> MEPSSKKLTGRLMLAVGGAVLGSLQFGYNTGVINAPQKVIEEFYNQTWVHRYGESILPTTLTTLWSLSVAIFSVGGMIGSFSVGLFVNRFGRRNSMLMMNLLAFVSAVLMGFSKLGKSFEMLILGRFIIGVYCGLTTGFVPMYVGEVSPTALRGALGTLHQLGIVVGILIAQVFGLDSIMGNKDLWPLLLSIIFIPALLQCIVLPFCPESPRFLLINRNEENRAKSVLKKLRGTADVTHDLQEMKEESRQMMREKKVTILELFRSPAYRQPILIAVVLQLSQQLSGINAVFYYSTSIFEKAGVQQPVYATIGSGIVNTAFTVVSLFVVERAGRRTLHLIGLAGMAGCAI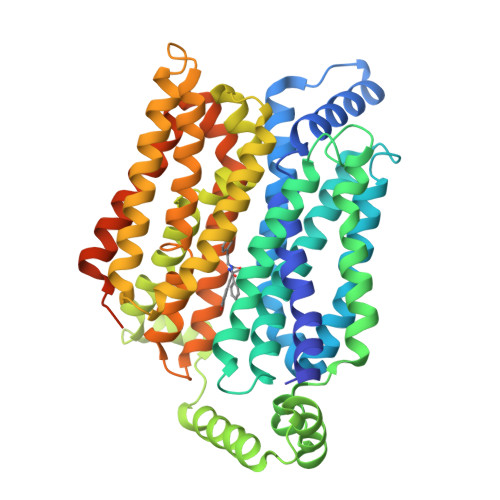LMTIALALLEQLPWMSYLSIVAIFGFVAFFEVGPGPIPWFIVAELFSQGPRPAAIAVAGFSNWTSNFIVGMCFQYVEQLCGPYVFIIFTVLLVLFFIFTYFKVPETKGRTFDEIASGFRQGGASQSDKTPEELFHPLGADSQV>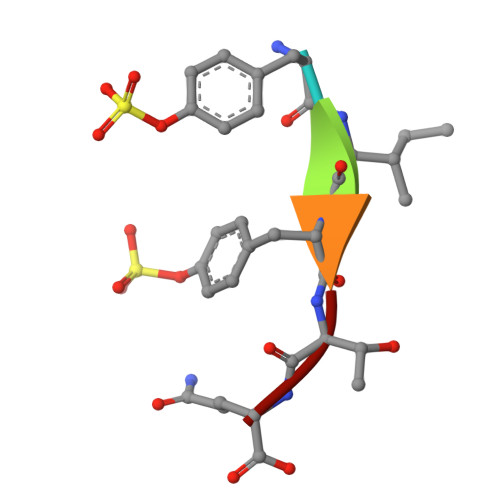 YIYTQ>CGC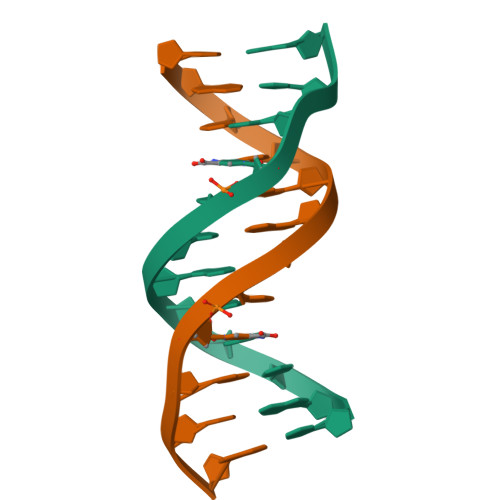GAATTXGCG[2x]> HEAEMKS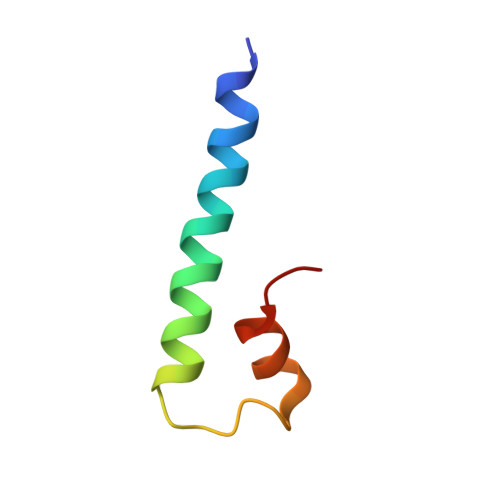NRRRWRIMKGAASAIVAGSGIDWVRDERLRDLVLDLPD4-{[5-fluoro-4-(3-{[(3R)-3-hydroxypyrrolidin-1-yl]methyl}-4-methyl-1H-pyrrol-1-yl)pyrimidin-2-yl]amino}-2,6-dimethylphenyl 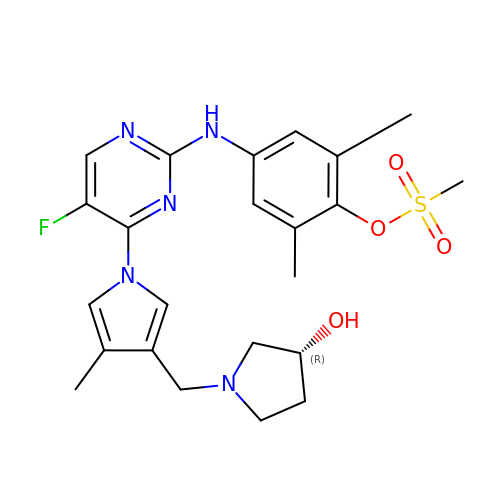methanesulfonate | C23 H28 F N5 O4 S | JEDIVKVRGQEZRX-LJQANCHMSA-N>MASGSNVEEYELDVEALVVILRDRNIPRNPLHGEVIGLRLTEGWWGQIERFQMVRLILQNDDNEPLQRPRYEVIQRAVNPHTMFMISGPLAELQLAFQDLDLPEGPLRFGPLANGHYVQGDPYSSSYRPVTMAETAQMTRDELEDVLNTQSEIEIQMINLLELYEVETRALRRQLAERSSTGQGGISPGAPRSRPPVSSFSGLPSLPSIPGIHPRAPSPPRATSTPGNIPWSLGDDNPPSSSFPGPSQPRVSFHPGNPFVEEEGHRPRSQSRERRREILPAPVPSAPPMIQYIPVPPPPPIGTVIPIQHIRSVTGEPPRNPREIPIWLGRNAPAIDGVFPVTTPDLRCRIINAILGGNIGLSLTPGDCLTWDSAVATLFIRTHGTFPMHQLGNVIKGIVDQEGVATAYTLGMMLSGQNYQLVSGIIRGYLPGQAVVTALQQRLDQEIDDQTRAETFIQHLNAVYEILGLNARGQSIRASVTPQPRPSRGRGRGQNTSRPSQGPANSGRGRQRPASGQSNRGSSTQNQNQDNLNQGGYNLRPRTYQPQRYGGGRGRRWNDNTNNQESRPSDQGSQTPRPNQAGSGVRGNQSQTPRPAAGRGGRGNHNRNQRSSGAGDSRAVNTVTQSATSSTDESSSAVTA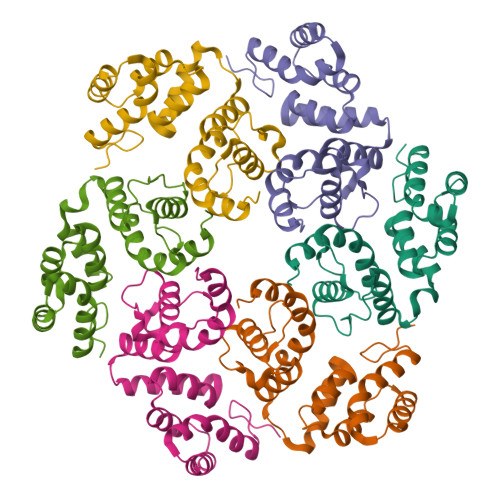ASGGDQRD[6x]> UGUUCUCU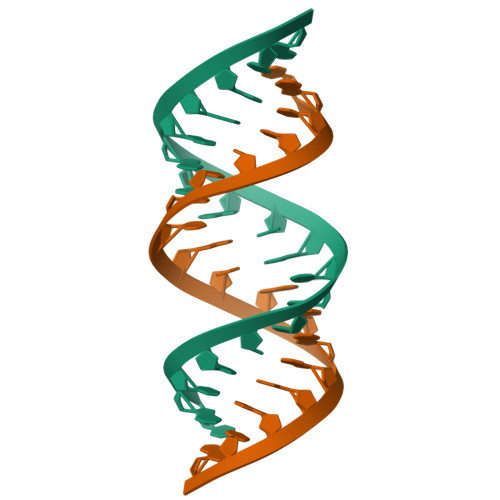ACGAAGAACA> VRPLNCIVAVSQNMGIGKNGDL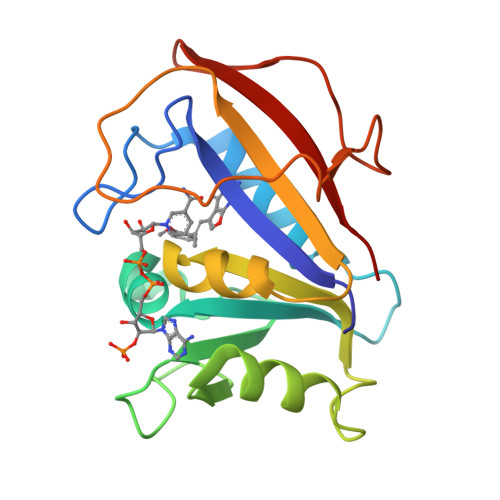PWPPLRNEFKYFQRMTTTSSVEGKQNLVIMGRKTWFSIPEKNRPLKDRINIVLSRELKEPPRGAHFLAKSLDDALRLIEQPELASKVDMVWIVGGSSVYQEAMNQPGHLRLFVTRIMQEFESDTFFPEIDLGKYKLLPEYPGVLSEVQEEKGIKYKFEVYEKKD5-butyl-8,8-dimethyl-3,6,8,9-tetrahydropyrazolo[3,4-b]thiopyrano[4,3-d]pyridin-1-amine | C15 H22 N4 S | 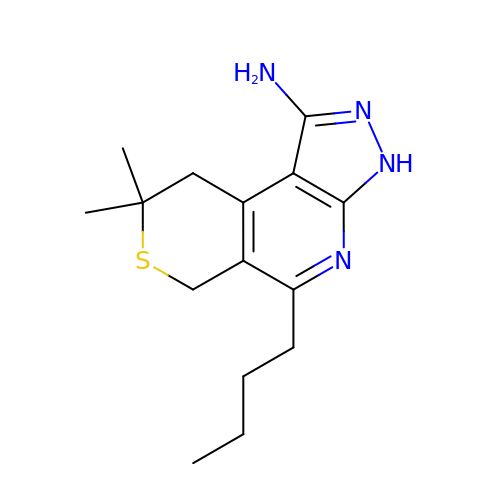MPWCUTPIYOWTII-UHFFFAOYSA-N> HHHHHHSGMKQLTILGSTGSIGCSTLDVVRHNPEHFRVVALVAGKNVTRMVEQCLEFSPRYAVMDDEASAKLLKTMLQQQGSRTEVLSGQQAACDMAALEDVDQVMAAIVGAAGLLPTLAAIRAGKTILLANK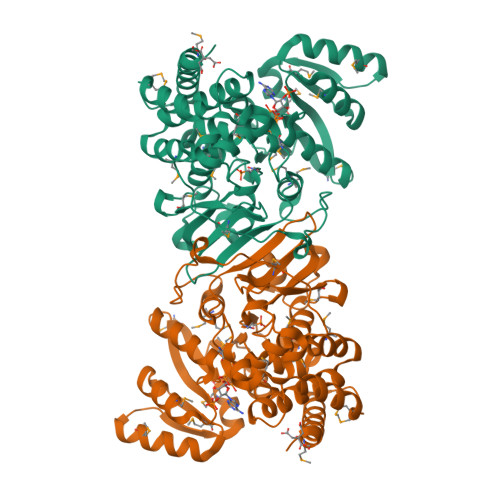ESLVTCGRLFMDAVKQSKAQLLPVDSEHNAIFQSLPQPIQHNLGYADLEQNGVVSILLTGSGGPFRETPLRDLATMTPDQACRHPNWSMGRKISVDSATMMNKGLEYIEARWLFNASASQMEVLIHPQSVIHSMVRYQDGSVLAQLGEPDMRTPIAHTMAWPNRVNSGVKPLDFCKLSALTFAAPDYDRYPCLKLAMEAFEQGQAATTALNAANEITVAAFLAQQIRFTDIAALNLSVLEKMDMREPQCVDDVLSVDANAREVARKEVMRLAS>[3x]MGQAGEITKYVNPFIGTGAIDGGLSGNNYPGATSPFGMIQLSPDTSEAPNWGDASGYDYNRNTIFGFSHTRLSGTGASDLIDITLMPTSSGRTSSAFTHDEEKARPGYYQVMLKDENINAELTTTQRNGIHRYQYPAGKDAEIILDMDHSADKGSWGRRIINSQIRILNDHAVEGYRIITGWAKLRKIYFYMEFSSPILTSTLRDGGRVHENTAVINGTNLHGCFRFGQLNGKPLTCKVALSSVSMENARQNMEQEAPHWDFDRYVAAADADWEKQLGKIEVKGTEVQKEIFYTALYHTMIQPNTMSDVNGEYMAADYTTRKVANNETHYTTFSLWDTFRASHPLYTLLEPERVTDFVKSMIRQYEYYGYLPIWQLWGQDNYCMIGNHSIPVITDAILKGIPGIDMEKAYEAVYNSSVTSHPNSPFEVWEKYGFMPENIQTQSVSITLEQAFDDWCVAQLAAKLNKDADYQRFHKRSEYYRNLFHPKTKFFQSKNDKGEWIEPFDPYQYGGNGGHPFTEGNAWQYFWYVPHNIQALMELTGGTKAFEQKLDTFFTSTYKSEQMNHNASGFVGQYAHGNEPSHHVAYLYNFAGQPWKTQKYVSHILNTLYNNTSSGYAGNDDCGQMSAWYVFSAMGFYPVNPADGRYIIGSPLLDECTLKLAGNKEFRIRTIRKSPEDIYIQSVTLNGKKHKDFFITHQDIMNGGTMVFKMGKKPSGWGKLEHHHHHH

Structural analyses of two glycoside hydrolase family 92 α-mannosidases, BT3130 and BT3965, together with mechanistically relevant complexes at 1.8–2.5 Å resolution reveal conservation of the global enzyme fold and core catalytic apparatus despite different linkage specificities. Most enzymes within family GH92 are exo-acting α-mannosidases that are capable of hydrolysing terminal mannosidic residues with a variety of linkages, including α-1,2, α-1,3, α-1,4 and α-1,6 glycosidic bonds. Complementary to α-mannosidases within largely eukaryotic mannosidase families (particularly GH38 and GH47) that play important roles in N-glycan processing, GH92 enzymes are metal-dependent, featuring a single Ca2+ ion coordinated within the catalytic active site. GH92 enzymes act via a classic single-displacement mechanism, leading to inverted configuration at the anomeric centre.

ManI is derived by the annulation of a deoxymannojirimycin piperidine ring with an imidazole, resulting in double-bond character between C1 and the endocyclic N atom, thus providing shape mimicry of the oxocarbenium ion-like character present at the TS‡ of glycosidase-catalysed hydrolysis. Therefore, to ensure observation of the true, catalytically competent forms of these enzymes, and the determination of meaningful ligand complexes, BT3130 was screened for crystallization with the addition of 10 mM calcium acetate (final concentation) to the protein buffer (in addition to avoiding K+-containing screen hits), while the subsequent ManI complexes of both enzymes were cryoprotected with the addition of 1 mM Ca2+ (final concentration) to the cryoprotectant solutions. Cofactor supplementation was successful, allowing determination of fully occupied enzyme–Ca2+–ManI complexes. Within the active site of BT3130, ManI is coordinated within a network of interactions: hydrogen bonding of O6 to the backbone amide of Gly92 (Gly70 in BT3965), hydrogen bonding of O4 to the side-chain N atom of Trp390 and Oδ2 of Asp353 (Trp383 and Asp344, respectively, in BT3965) and a hydrophobic stacking interaction with the side chain of Met400 (Met393 in BT3965), which is positioned directly beneath the plane of the sugar ring. The carboxylate side chain of Asp353 (Asp344 in BT3965) makes a bridging interaction, simultaneously binding to the inhibitor O3 and O4 positions. Remarkably, despite differing substrate specificities (BT3130 is characterized as uncertain linkage preference, with weak activity against α-1,3-mannobiose and strong activity against yeast α-mannan, while BT3965 is a highly active α-1,4-mannosidase; Zhu et al., 2010), all observed enzyme–inhibitor interactions within the −1 subsite of both proteins are fully conserved.> GHRP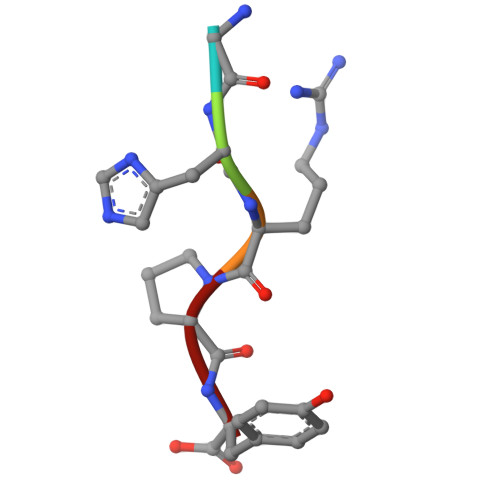Y> DQAGKSPAGVRYHGGDEIILQGFH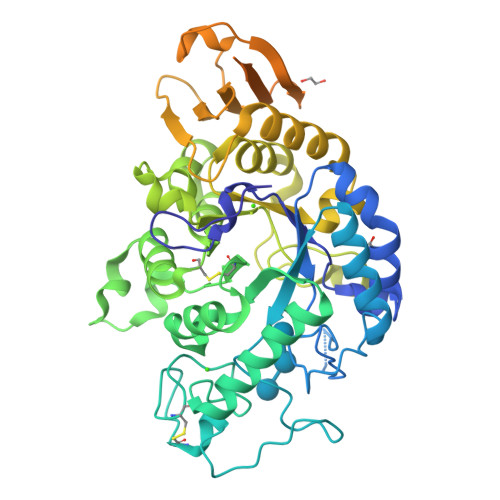WNVVREAPNDWYNILRQQASTIAADGFSAIWMPVPWRDFSSWTDGGKSGGGEGYFWHDFNKNGRYGSDAQLRQAAGALGGAGVKVLYDVVPNHMNRGYPDKEINLPAGQGFWRNDCADPGNYPNDCDDGDRFIGGESDLNTGHPQIYGMFRDELANLRSGYGAGGFRFDFVRGYAPERVNSWMTDSADSSFCVGELWKGPSEYPSWDWRNTASWQQIIKDWSDRAKCPVFDFALKERMQNGSVADWKHGLNGNPDPRWREVAVTFVDNHDTGYSPGQNGGQHHWALQDGLIRQAYAYILTSPGTPVVYWSHMYDWGYGDFIRQLIQVRRTAGVRADSAISFHSGYSGLVATVSGSQQTLVVALNSDLANPGQVASGSFSEAVNASNGQVRVWRSGSGDGGGNDGGEGGLVNVNFRCDNGVTQMGDSVYAVGNVSQLGNWSPASAVRLTDTSSYPTWKGSIALPDGQNVEWKCLIRNEADATLVRQWQSGGNNQVQAAAGASTSGSF>[4x]MEKDLQLRVNEKLDVENILKDLDKYTPKRRGWTWRQPAENLQMGPFIYKDASTPLENSVALPSAKYFGDIDPQPLPVITTEIASGRFEDDIRRMRMAAWHGADHIMVIRTAGQSHYDGLIEGTPQGIGGVPITRKQVRAQRKALDLIEEEVGRPINYHSYVSGVAGPDIAVMFAEEGVNGAHQDPQYNVLYRNINMIRSFIDACESKTIMAWADMAQIDGAHNANATAREAWKVMPELMVQHALNSI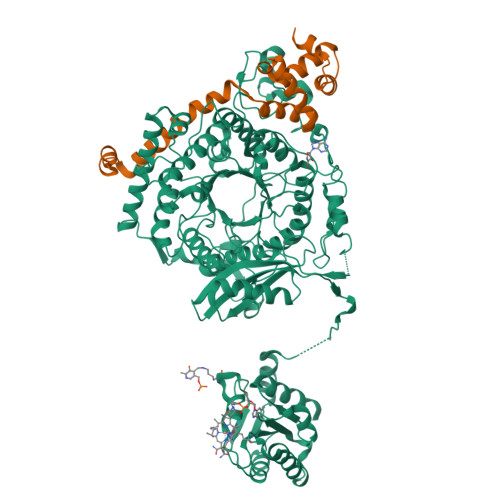FSLKVGMKKSNICLSTVPPTAPPAPSMYLDLPYAVALREMFEGYRMRAQMNTKYMEASTREATVTHVLNLLISKLTRADIQSTITPDEGRNVPWHIYNIEACDTAKQALIGMDGLMDMVQLKREGVLGDTVRELKERAVLFMEEIIEAGGYFNAVEQGFFVDSGYYPERNGDGIARQINGGIGAGTVFERDEDYMAPVTAHFGYNNVKQYDEALVSEPSKLIDGCTLEVPEKIVYIDELDENDNVNVRMEETKEFRHSSMIKPEVEWQADGTVLLTMFLPTSKRVAEFAAIEFAKKMNLEEVEVINREVMQEAEGTRIELKGRVPFSIDINSLVIPPEPEILSEDEIREDIEKTPLKIVAATVGEDEHSVGLREVIDIKHGGIEKYGVEVHYLGTSVPVEKLVDAAIELKADAILASTIISHDDIHYKNMKRIHELAVEKGIRDKIMIGCGGTQVTPEVAVKQGVDAGFGRGSKGIHVATFLVKKRREMREGKSEDPNSSSVDKLAAALEHHHHHH;>MKRADDFQQRRAHLANLSDEELQTRFWEMAEKIVDPLLDLGKKNTTPSIERSVLLRMGFSSLEAKAIVDKTMDRGLMGKGAGHIVYKIAKEKNISVREAGLALSEGKYWDDAIQIFKGGVK[4x]Herpesviruses cause severe diseases particularly in immunocompromised patients. Both genome packaging and release from the capsid require a unique portal channel occupying one of the 12 capsid vertices. Recent symmetry-relaxed cryo-EM reconstruction strategies of α- and γ-herpesviral virions provided first snapshots of the unique portal vertex that is essential for DNA encapsidation and release. These studies revealed for the first time a pentameric cap on top of the portal that presumably seals the capsids against DNA leakage after packaging and has been proposed to consist of pUL25 in HSV-1 and its ortholog pORF19 in KSHV. Here, we report the crystal structures of the CTDs of pUL25 orthologs from 3 members of the β- and γ-herpesviruses (HCMV, KSHV, and murid gammaherpesvirus 68 (MuHV-68)), highlighting their structural conservation across the herpesvirus subfamilies. The overall structures of the HSV-1, HCMV, KSHV, and MuHV-68 orthologs are well conserved as reflected by high z scores resulting from structural comparisons using the Dali server and in spite of a low amino acid identity within the “twilight zone” (approximately 20% between the crystallized fragments of HSV-1 pUL25 and MuHV-68 pORF19; illustrated in the structural alignment in S3 Fig).

By contrast, pORF19KCTD assembled as pentamers in 3 independent crystal forms with either a single pentamer or 2 pentamers per asymmetric unit. The pentamer has an outer diameter of approximately 142 Å, a central cavity of approximately 14 Å that is slightly narrower than the diameter of a double-stranded DNA helix (approximately 20 Å) and lateral interactions that bury an area of approximately 1,049 Å2 (±44.5 Å2) on one protomer and approximately 1,147 Å2 (±53.1 Å2) on the adjacent protomer. An extensive interaction network consisting of hydrophobic interactions, hydrogen bonds, and a salt bridge stabilizes this interface, and its calculated total binding energy amounts to approximately 19.2 kcal/mol (±0.9 kcal/mol). The protomers also interact via an intermolecular β-sheet formed by a surface loop (residues 454 to 467) comprising a short β-strand (residues 462 to 464), which runs parallel to an N-terminal 2-stranded β-sheet of the adjacent protomer. These inter-protomer main chain β-interactions are likely to confer extra stability to the pentamer. Our crystal structure also reveals that each protomer binds 2 acetate ions via 4 intra-protomeric hydrogen bonds (acetate622) and 3 salt bridges (acetate623), respectively. One of these acetate ions (acetate623) connects 2 adjacent protomers via polar interactions with the side chain of Gln458 of the adjacent protomer, thereby further stabilizing the pentameric interactions.

>MASHRNFTVAIVPGDPHFSVDRDLRGELMPTLYMNQNQWLPSFGPWFISLTDNAMQRRVFPKELKGTVNFQNSTSLKLISHTLTTVASTTADFFADARHLTDTQAALCLVNAYFCQKTSRQLPATPDDLLADLPQKLDLLITQLKQESGPGDFSFTYSNPQERASLAPLNKESRYPTAFFQRHKLHAMMAKAGLFPHNKGTGAPGTAPAMDLVFAITSAMFGSDIPPFSAYQWNLRAGIVALEVFILAYGLLEFGQVARGHPNRRLNLVSLLGPKFQPGALPDPNAPMLKRGQLFSFISEHYIIPTLQANPNAPVSFIFPGIILAALEARSTVSHKQPGPFVNLTGSRFNEIFEILNQQLTFRDPLALLQARTALRLATEEGLDVLLSHPSPPTLLQEIIKSQFGGGDDYDRAYFMVLGCLPVVLAVVPAAALEHHHHHHHHH[10x]> RLSLQNTAEIQHCLVNAGDVGCGVFECFENNSCEIRGLHGICMTFLHNAGKFDAQGKSFIKDALKCKAHALRHRFGCISRKCPAIREMVSQLQRECYLKHDLCAAAQENTRVIVEMIHFKDLLLHEPYVDLVNLLLTCGEEVKEAITHSVQVQCEQNWGSLCSILS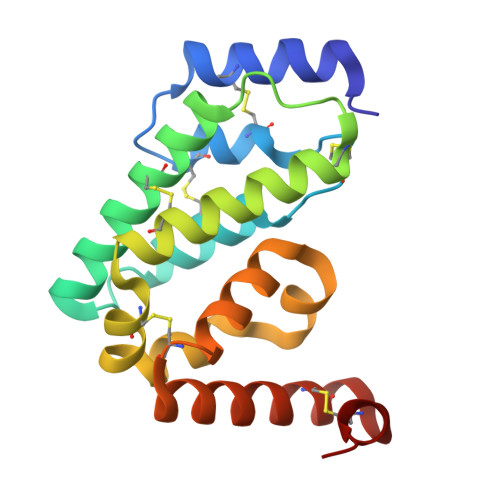FC> MGPVWRKHYITYRINNYTPDMNREDVDYAIRKAFQVWSNVTPLKFSKINTGMADILVVFARGAHGDDHAFDGKGGILAHAFGPGSGIGGDAHFDEDEFWTTHSGGTNLF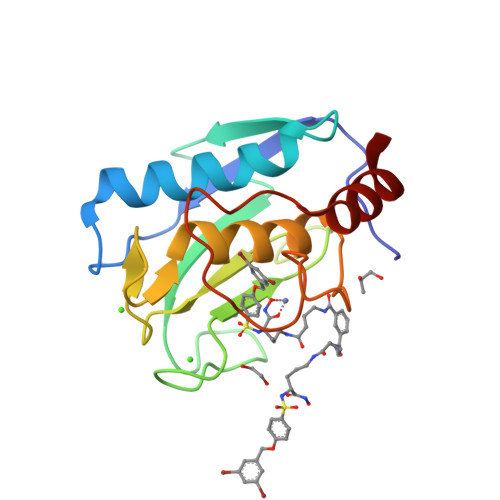LTAVHEIGHSLGLGHSSDPKAVMFPTYKYVDINTFRLSADDIRGIQSLYG> MVQYIFTPWRNRAELLAVRAQFYPEHTSKTHLKKHHQSTFQDDEHIRSEKQKAVARVSMWMQRGGCPHMVESTALLVAAILSDEAQGSGAAGGYAVRAAYSAAFSR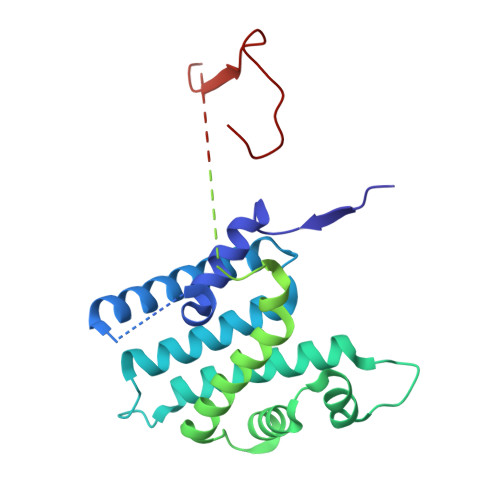FVTGLLDSHQDKQRKQSMYDVAKAVGLPAAFVELRHQATHEQLPSLTRLRSAARRALEWIWWYYWKGLGPVDMVQRGVNGKGVAGVGDTSESEEKDVGEEGGDAAARCREGVVRLLESDVRVGGEAINGPGKEELLAEFGEALVLTTLDAAAGNTRDVGVLRRAIGLMREIVNGGDEDCMQLENGKGNRDVEKLKEELKKGWEEIKRLAQEKEDSGDDQTEDEDVDMEAEEEDKKEQQSGWVLYDEKEWVPKPIGIV>TLNESLQTEKFDFGTMVQWAYDHKYAEESKIAYEYALAAGSDSNARAFLATNSQAKHVKDCATMVRHYLRAETQALSMPAYIKARCKLATGEGSWKSILTFFNYQNIELITFINALKLWLKGIPKKNCLAFIGPPNTGKSMLCNSLIHFLGGSVLSFANHKSHFWLASLADTRAALVDDATHACWRYFDTYLRNALDGYPVSIDRKHKAAVQIKAPPLLVTSNIDVQAEDRYLYLHSRVQTFRFEQPCTDESGEQPFNITDADWKSFFV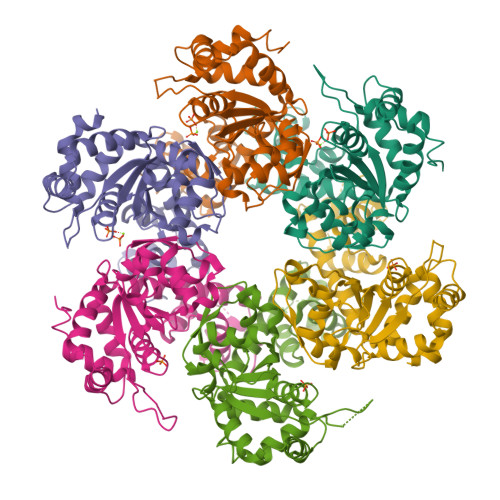RLWGRLDLIDEEEDSEEDGDSMRTFTCSARNTNAVD[6x]> SMTGGQQMGRGSMDITMFKEDLKSHLEEKIIPFWQSLKDDEFGGYYGYMDFNLNIDRKAQKGCVLNSRILWFFSACYNVLKSEKCKEMAFHAFEFLKNKFWDKEYEGLFWSVSHKGVPVDVTKHVYVQAFGIYGLSEYYEASGDEEALHMAKRLFEILETKCKRENGYTEQFERNWQEKENRFLSENGVIASKTMNTHLHVLESYTNLYRLLKLDDVYEALEWIVRLFVDKIYKKGTGHFKVLCDDNWNELIKAVSYGHDIEASWLLDQAAKYLKDEKLKEEVEKLALEVAQITLKEAFDGQSLINEMIEDRIDRSK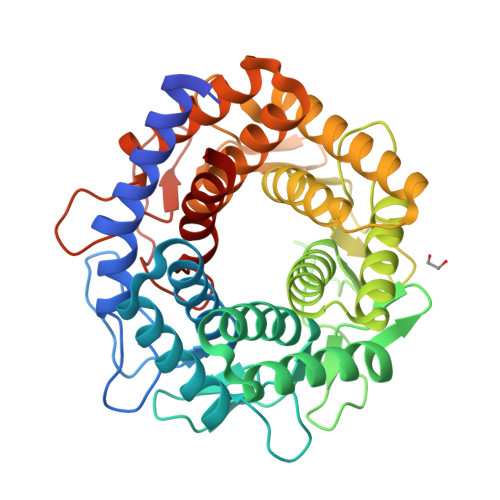IWWVEAETVVGFFNAYQKTKEEIYLDAAIKTWEFIKEHLVDRRKNSEWLWKVNEDLEAVNMPIVEQWKCPYHNGRMCLEIIKRVD> MGSSHHHHHHSQDPNSVRLAEELERQQLLEKRKKERNLHLQKINSIIDFIKERQSEQWSRQERCFQFGRLGASLHNQMEKDEQKRIEKTAKQRLAALKSNDEEAYLKLLDQTKDTRITQLLRQTNSFLDSLSEAVRAQQNEAKILHGEEVQPITDEEREKTDYYEVAHRIKEKIDKQPSILVGGTLKEYQLRGLEWMVSLYNNHLNGILADEMGLGKTIQSISLITYLYEVKKDIGPFLVIVPLSTITNWTLEFEKWAPSLNTIIYKGTPNQRHSLQ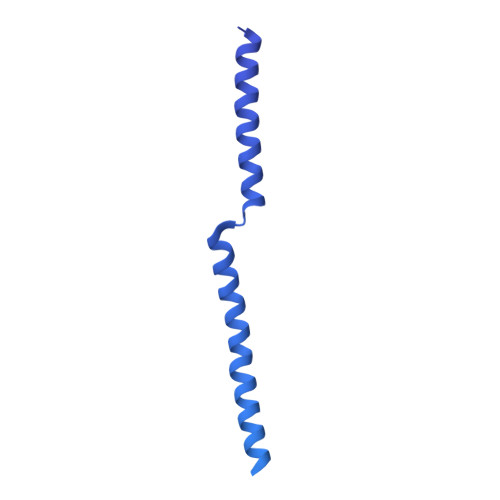HQIRVGNFDVLLTTYEYIIKDKSLLSKHDWAHMIIDEGHRMKNAQSKLSFTISHYYRTRNRLILTGTPLQNNLPELWALLNFVLPKIFNSAKTFEDWFNTPFANTGTQEKLELTEEETLLIIRRLHKVLRPFLLRRLKKEVEKDLPDKVEKVIKCKLSGLQQQLYQQMLKHNALFVGAGTEGATKGGIKGLNNKIMQLRKICNHPFVFDEVEGVVNPSRGNSDLLFRVAGKFELLDRVLPKFKASGHRVLMFFQMTQVMDIMEDFLRMKDLKYMRLDGSTKTEERTEMLNAFNAPDSDYFCFLLSTRAGGLGLNLQTADTVIIFDTDWNPHQDLQAQDRAHRIGQKNEVRILRLITTDSVEEVILERAMQKLDIDGKVIQAGKFDNKSTAEEQEAFLRRLIESETNRDDDDKAELDDDELNDTLARSADEKILFDKIDKERMNQERADAKAQGLRVPPPRLIQLDELPKVFREDIEEHFKKEDSEPLGRIRQKKRVYYDDGLTEEQFLEAVEDDNMSLEDAIKKRREARERRRLRQ>[2x]YGTQIAEITAREILDSRGRPTVEAEVHLEDG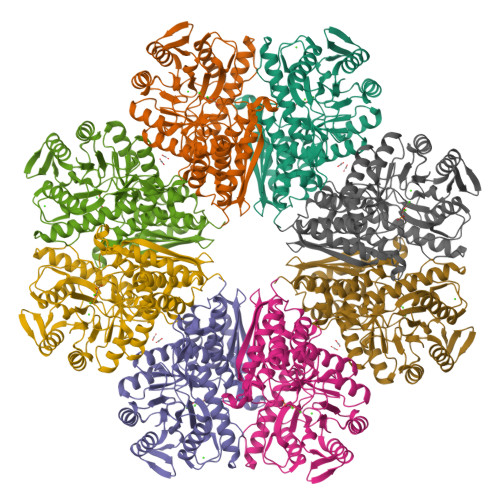SVGLAQVPSGASTGTFEAHELRDDDPSRYGGKGVQKAVENVSAIEDALIGLSALDQEGLDKAMIALDGTPNKKNLGANAILAVSLATAHAAATSLNLPLYRYLGGPLANVLPVPMMNVINGGAHADNNVDFQEFMIMPVGAPSFKEALRWGAEVFHALAKVLKDKGLATGVGDEGGFAPNLGSNKEALELLLTAIEAAGYKPGEQVALAMDVASSEFYKNGLYTCDGVSHEPAGMIGILADLVSQYPIVSIEDGLQEDDWSNWKTLTQQLGSTVQLVGDDLFVTNPDRLQSGIEQGVGNAVLIKLNQIGTLTETLRTIDLATRSGYRSVISHRSGETEDTTIADLAVATRAGQIKTGSLSRSERIAKYNRLLRIEAALGENALYAGAIGLGPK>[3x]MHHHHHHTQHGIRLPLRS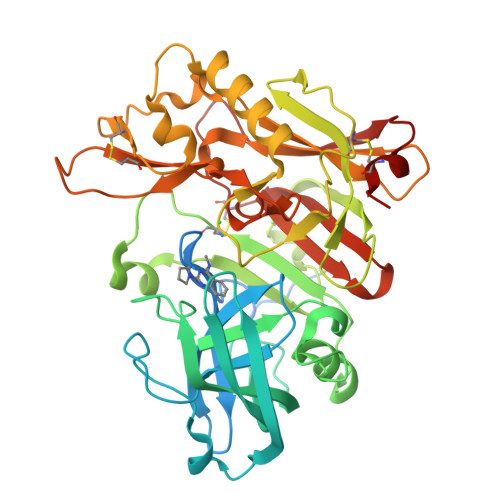GLGGAPLGLRLPRETDEEPEEPGTTGSFVEMVDNLRGKSGQGYYVEMTVGSPPQTLNILVDTGSSNFAVGAAPHPFLHRYYQRQLSSTYRDLRKGVYVPYTQGKWEGELGTDLVSIPHGPNVTVRANIAAITESDKFFINGSNWEGILGLAYAEIARPDDSLEPFFDSLVKQTHVPNLFSLQLCGAGFPLNQSEVLASVGGSMIIGGIDHSLYTGSLWYTPIRREWYYEVIIVRVEINGQDLKMDCKEYNYDKSIVDSGTTNLRLPKKVFEAAVKSIKAASSTEKFPDGFWLGEQLVCWQAGTTPWNIFPVISLYLMGEVTNQSFRITILPQQYLRPVEDVATSQDDCYKFAISQSSTGTVMGAVIMEGFYVVFDRARKRIGFAVSACHVHDEFRTAAVEGPFVTLDMEDCGYN In previous work we have explored the potential for establishing a bump-&-hole system targeting the bromodomains of the BET (bromo and extra-terminal) protein family. These four human proteins – BRD2, BRD3, BRD4 and BRDT – each contain two tandem bromodomains that bind acetylated lysine residues in histone tails, leading to the recruitment of multi-protein complexes to chromatin. Through this function the BET proteins play a significant role in controlling transcription and regulating gene expression. The phenotypes generated by said inhibitors have been used to investigate the functions of BET proteins and their significance as therapeutic targets. This process has been limited by the pan-selective nature of the BET inhibitors, as they typically target all BET bromodomains with similar potency, hence specific proteins/bromodomains cannot be associated to specific phenotypes. Through structural analysis of the bromodomain we hypothesized that a leucine/valine substitution (L/V) would be a more conservative change than the previous L/A substitution, resulting in a smaller ‘hole’ but still allowing enough space to accommodate a bumped ligand.

First, to cover a range of bump sizes, we included primary alkyl methyl, ethyl and propyl as well as allyl ‘bump’ modifications. With larger bumps, however, the rotational flexibility of the bump becomes important, with the semi-rigid 5 bump acting more like the equally flexible 4 bump than the 6 bump of similar length. Co-crystal structures of BRD2 BD2 L/V bound to 5 and 24 show that the tert-butyl group clashes with Leu381, reducing L/V potency. As this clash pushes the ligand away from the ZA loop it may relieve the bump/leucine steric clash and increase WT potency. The following compounds met the selection criteria for both the AlphaLISA assay and DMPK triage and hence underwent ITC profiling: 4, 5, 7, 8, 16, 17 and 21.

>[4x]SMGKLSEQLKHCNGILKELLSKKHAAYAWPFYKPVDASALGVHDYHDIIKHPMDLSTVKRKMENRDYRDAQEFAADVRLMFSNCYKYNPPDHDVVAMARKLQDVFEFRYAKMPD>MTEMTKPFLIVIVGPTASGKTELSIEVAKKFNGEIISGDSMQVYQGMDIGTAKVTTEEMEGIPHYMIDILPPDASFSAYEFKKRAEKYIKDITRRGKVPIIAGGTGLYIQSLLYNYAFEDESISEDKMKQVKLKLKELEHLNNNKLHEYLASFDKESAKDIHPNNRKRVLRAIEYYLKTKKLLSSRKKVQQFTENYDTLLIGIEMSRETLYLRINKRVDIMLGHGLFNEVQHLVEQGFEASQSMQAIGYKELVPVIKGNI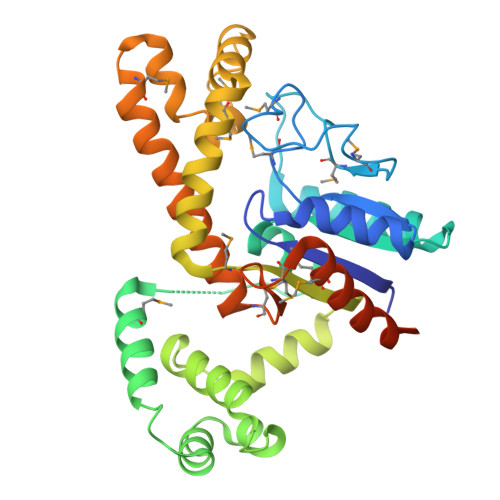SMENAVEKLKQHSRQYAKRQLTWFKNKMNVHWLNKERMSLQMMLDEITTQINKRSSNHDCKRKHPRPSTRELLEHHHHHH[2x]>[4x]MSRHWPLFDLRITTPRLQLQLPTEELCDQLIDTILEGVHDPDRMPFSVPWTRASREDLPFNTLSHLWQQLAGFKRDDWSLPLAVLVDGRA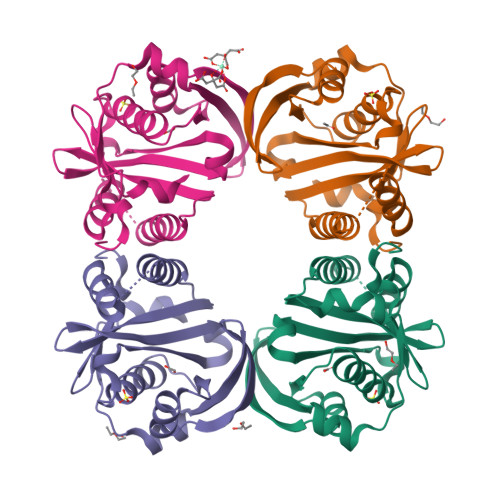VGVQALSSKDFPITRQVDSGSWLGLRYQGHGYGTEMRAAVLYFAFAELEAQVATSRSFVDNPASIAVSRRNGYRDNGLDRVAREGAMAEALLFRLTRDDWQRHRTVEVRVDGFDRCRPLFGPLEPPRY(3R)-3-hydroxybutanoic acid | C4 H8 O3 | 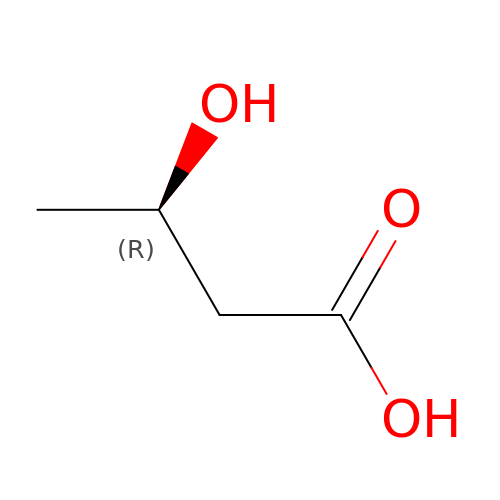WHBMMWSBFZVSSR-GSVOUGTGSA-N>SKKVIVIAGTTGVGKSQLSIQLAQKFNGEVINSDSMQVYKDIPIITNKHPLQEREGIPHHVMNHVDWSEEYYSHRFETECMNAIEDIHRRGKIPIVVGGTHYYLQTLFNKRVDTKSSERKLTRKQLDILESTDPDVIYNTLVKCDPDIATKYHPNDYRRVQRMLEIYY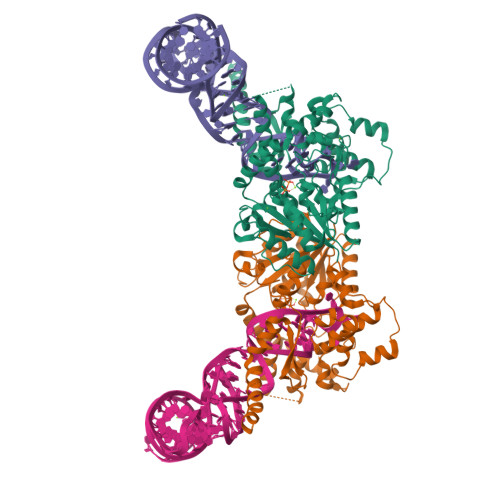KTGKKPSETFNEQKITLKFDTLFLWLYSKPEPLFQRLDDRVDDMLERGALQEIKQLYEYYSQNKFTPEQCENGVWQVIGFKEFLPWLTGKTDDNTVKLEDCIERMKTRTRQYAKRQVKWIKKMLIPDIKGDIYLLDATDLSQWDTNASQRAIAISNDFISNRPIKQERAPKALEELLSKGETTMKKLDDWTHYTCNVCRNADGKNVVAIGEKYWKIHLGSRRHKSNLKRNTRQADFEKWKI[2x]> RTIVVTTILESPYVMYKKNHEQLEGNERYEGYCVDLAYEIAKHVRIKYKLSIVGD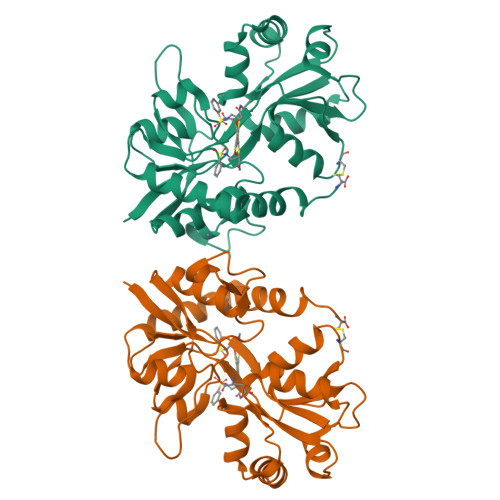GKYGARDPETKIWNGMVGELVYGRADIAVAPLTITLVREEVIDFSKPFMSLGISIMIKKGTPIESAEDLAKQTEIAYGTLDSGSTKEFFRRSKIAVYEKMWSYMKSAEPSVFTKTTADGVARVRKSKGKFAFLLESTMNEYIEQRKPCDTMKVGGNLDSKGYGVATPKGSALGNAVNLAVLKLNEQGLLDKLKNKWWYDKGEC> MTTAAGLSGIDLTDLDNFADGFPHHLFAIHRREAPVYWHRPTEHTPDGEGFWSVATYAETLEVLRDPVTYSSVTGGQRRFGGTVLQDLPVAGQVLNMMDDPRHTRIRRLVSSGLTPRMIRRVEDDLRRRARGLLDGVEPGAPFDFVVEIAAELPMQMICILLG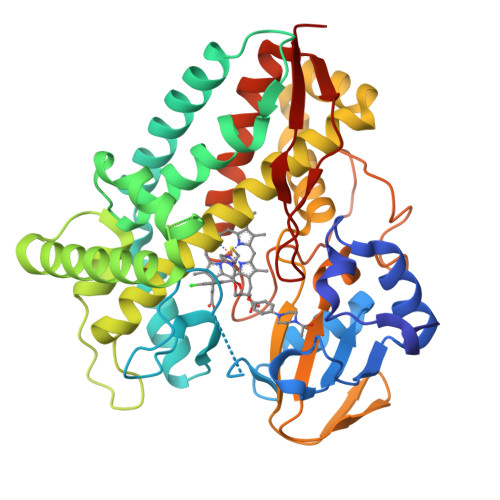VPETDRHWLFEAVEPGFDFRGSRRATMPRLNVEDAGSRLYTYALELIAGKRAEPADDMLSVVANATIDDPDAPALSDAELYLFFHLLFSAGAETTRNSIAGGLLALAENPDQLQTLRSDFELLPTAIEEIVRWTSPSPSKRRTASRAVSLGGQPIEAGQKVVVWEGSANRDPSVFDRADEFDITRKPNPHLGFGQGVHYCLGANLARLELRVLFEELLSRFGSVRVVEPAEWTRSNRHTGIRHLVVELRGG> MEHQLLCCEVETIRRAYPDANLLNDRVLRAMLKAEETCAPSVSYFKCVQKEVLPSMRKIVATWMLEVCEEQKCEEEVFPLAMNYLDRFLSLEPVKKSRLQLLGATCMFVASKMKETIPLTAEKLCIYTDNSIRPEELLQMELLLVNKLKWNLAAMTPHDFIEHFLSKMPEAEENKQIIRKHAQTFVALCATDVKFISNPPSMVAAGSVVAAVQGLNLRSPNNFLSYYRLTRFLSRVIKCDPDCLRACQEQIEALLESSLRQAQQNMDPKAA;> MATSRYEPVAEIGVGAYGTVYKARDPHSGHFVALKSVRVPNGEEGLPISTVREVALLRRLEAFEHPNVVRLMDVCATSRTDREIKVTLVFEHVDQDLRTYLDK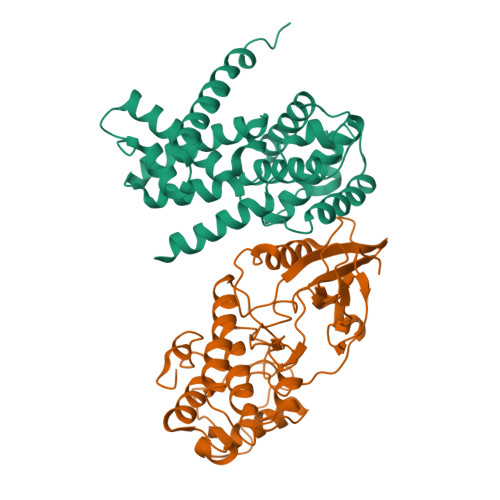APPPGLPAETIKDLMRQFLRGLDFLHANCIVHRDLKPENILVTSGGTVKLADFGLARIYSYQMALAPVVVTLWYRAPEVLLQSTYATPVDMWSVGCIFAEMFRRKPLFCGNSEADQLGKIFDLIGLPPEDDWPRDVSLPRGAFPPRGPRPVQSVVPEMEESGAQLLLEMLTFNPHKRISAFRALQHSYLHKDEGNPEHHHHHH>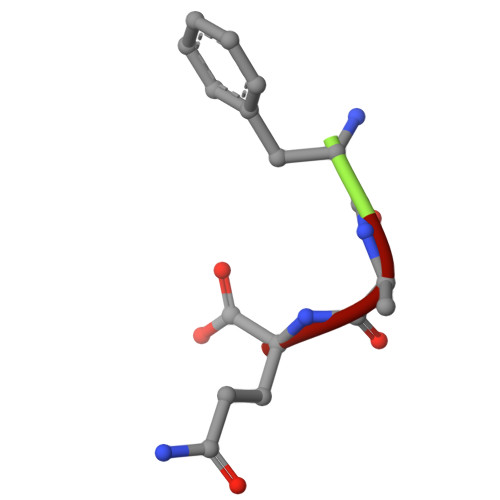 FAQ> AECSVDIQGNDQMQFNTNAITVDKSCKQFTVNLSHPGNLPKNVMGHSWVLSTAADMQGVVTDGMASGLDKDYLKPDDSRVIAHTK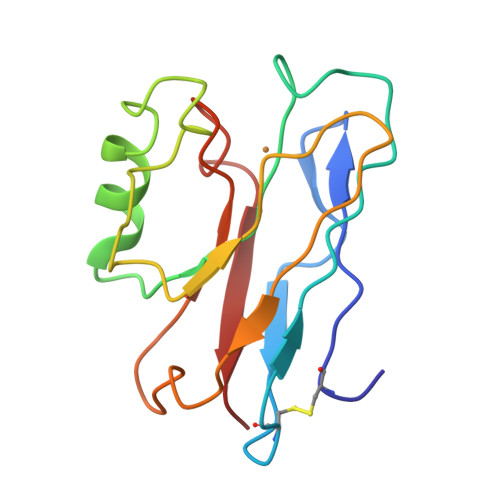LIGSGEKDSVTFDVSKLKEGEQYMFFCTFPGHSALLKGTLTLK> SIQVTPRSIVINRMNNIQINPTSIGNPNNGLHMTYNNAAAAAAAAAAAAAAAAAAAAAAAAAAAAAAAASIQVTPRSIVINRMNNIQINPTSIGNPQVTIRLPLNNFKSTTQLIQQVSLTDFFRPDIEHAGSTVLILRHPTDLPAL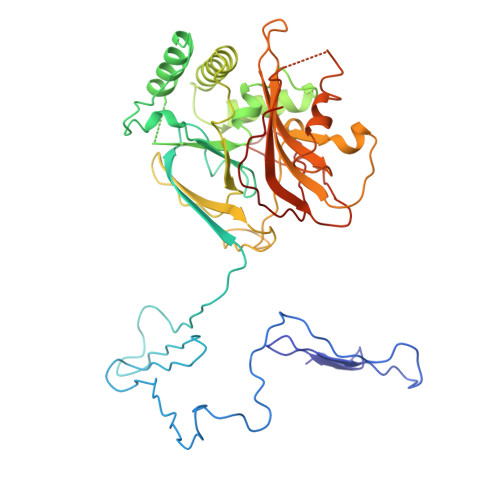ARHRAPPGRQTERLAEAWGQLLEASRAYVTSLSFIAACRAEEYTDKQAAEANRTAIVSAYGCSRMGARLIRFSECLRAMVQCHVFPHRFISFFGSLLEYTIQDNLCNITAVAKGPQEAARTDKTSTRRVTANIPACVFWDVDKDLHLSADGLKHVFLVFVYTQRRQREGVRLHLALSQLNEQCFGRGIGFLLGARICMYAAYTLIGTIPSESVRYTRRMERFGGYNVPTIWLEGVVWGGTNTWNEC>[4x]THPDISVDVLVIGAGPTGLGAAKRLNQIDGPSWMIVDSNETPGGLASTDVTPEGFLYDVGGHVIFSHYKYFDDCLDEALPKEDDWYTHQRISYVRCQGQWVPYPFQNNISMLPKEEQVKCIDGMIDAAL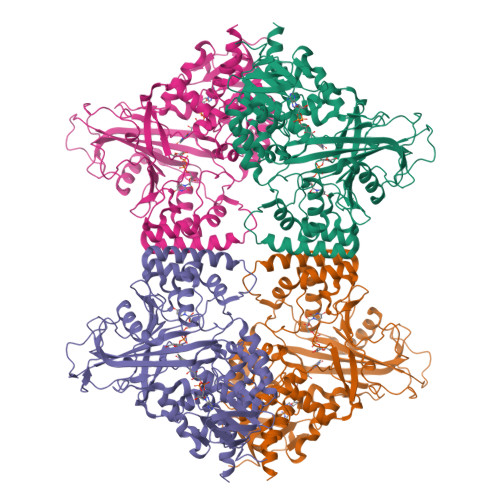EARVANTKPKTFDEWIVRMMGTGIADLFMRPYNFKVWAVPTTKMQCAWLGERVAAPNLKAVTTNVILGKTAGNWGPNATFRFPARGGTGGIWIAVANTLPKEKTRFGEKGKVTKVNANNKTVTLQDGTTIGYKKLVSTMAVDFLAEAMNDQELVGLTKQLFYSSTHVIGVGVRGSRPERIGDKCWLYFPEDNCPFYKATIFSNYSPYNQPEASKKLPTMQLADGSRPQSTEAKEGPYWSIMLEVSESSMKPVNQETILADCIQGLVNTEMLKPTDEIVSTYHRRFDHGYPTPTLEREGALTQILPKLQDKDIWSRGRFGSWRYEVGNQDHSFMLGVEAVDNIVNGAVELTLNYPDFVNGRQNTERRLVDGAQVFAKSKAQL>GMEYQLQQLASLTLVGIKETYENGRQAQQHIAGFWQRCYQEGVIADLQLKNNGDLAGILGLCIPELDGKMSYMIAVTGDNSADIAKYDVITLASSKYMVFEAQGAVPKAVQQKMEEVHHY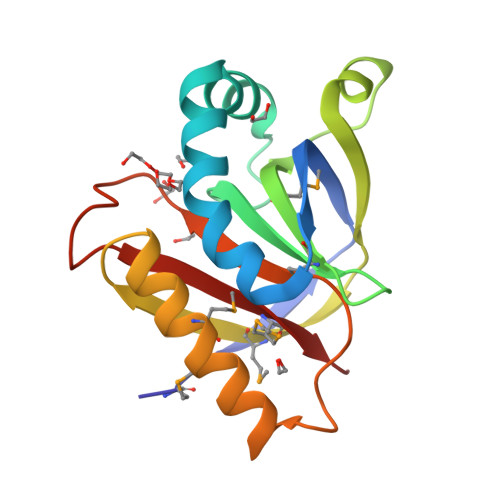IHQYQANTVKSAPFFELYQDGDTTSEKYITEIWMPVKG[3x]>GPGNEVTLLDSRSVQGELGWIASPLEGGWEEVSIMDEKNTPIRTYQVCNVMEPSQNNWLRTDWITREGAQRVYIEIKFTLRDCNSLPGVMGTCKETFNLYYYESDNDKERFIRENQFVKIDTIAADESFTQVDIGDRIMKLNTEIRDVGP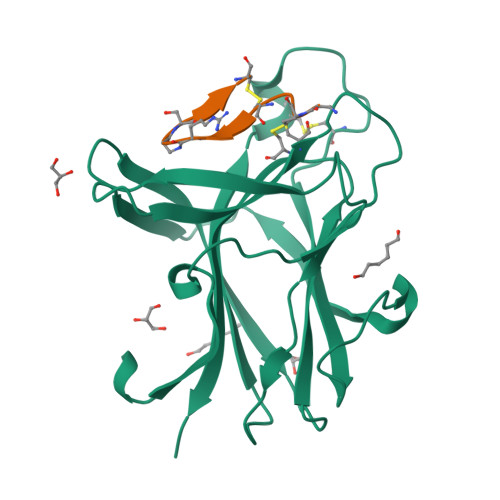LSKKGFYLAFQDVGACIALVSVRVFYKKA[4x]> APQFFNIID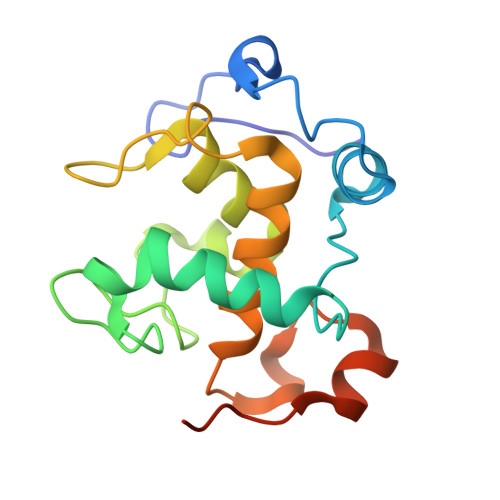GSPLNFDDAMEEGRDTEAVKHFLETGENVYNEDPEILPEAEELYAGMCSGCHGHYAEGKIGPGLNDAYWTYPGNETDVGLFSTLYGGATGQMGPMWGSLTLDEMLRTMAWVRHLYTGDPKDASWLTDEQKAGFTPFQPKSSGEDQS>[48x]MGMQGDPDVLRLLNEQLTSELTAINQYFLHSKMQDNWGFTELAAHTRAESFDEMRHAEEITDRILLLDGLPNYQRIGSLRIGQTLREQFEADLAIEYDVLNRLKPGIVMC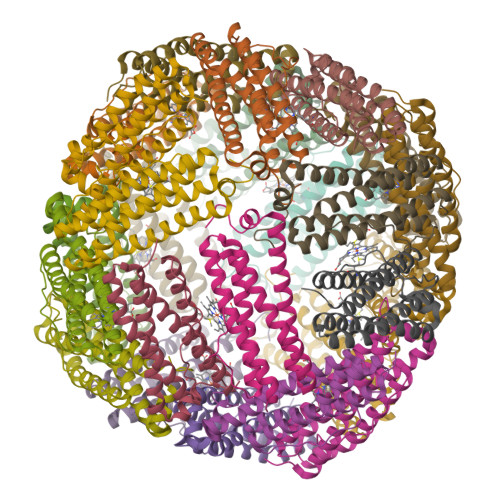REKQDTTSAVLLEKIVADEEEHIDYLETQLELMDKLGEELYSAQCVSRPPT> DPDTAVTNKQSFSTDVIYQVFTDRFLDGNPSNNPTGAAYDATCSNLKLYCGGDWQGLINKINDNYFSDLGVTALWISQPVENIFATINYSGVTNTAYHGYWARDFKKTNPYFGTMADFQNLITTAHAKGIKIVIDFAPNHTSPAMETDTSFAENGRLYDNGTLVGGYTNDTNGYFHHNGGSDFSSLENGIYKNLYDLADFNHNNATIDKYFKDAIKLWLDMGVDGIRVAAVKHMPLGWQKSWMSSIYAHKPVFTFGEWFLGSAASDADNTDFANKSGMSLLDFRFNSAVRNVFRDNTSNMYALDSMINSTATDYNQVNDQVTFIDNHDMDRFKTSAVNNRRLEQALAFTLTSRGVPAIYYGTEQYLTGNGDPDNRAKMPSFSKSTTAFNVISKLAPLRKSNPAIAYGSTQQRWINNDVYVYERKFGKSVAVVAVNRNLSTSASITGLSTSLPTGSYTDVLGGVLNGNNITSTNGSINNFTLAAGATAVWQYTTAETTPTIGHVGPVMGKPGNVVTIDGRGFGSTKGTVYFGTTAVTGAAITSWEDTQIKVTIPSVAAGNYAVKVAASGVNSNAYNNFTILTGDQVTVRFVVN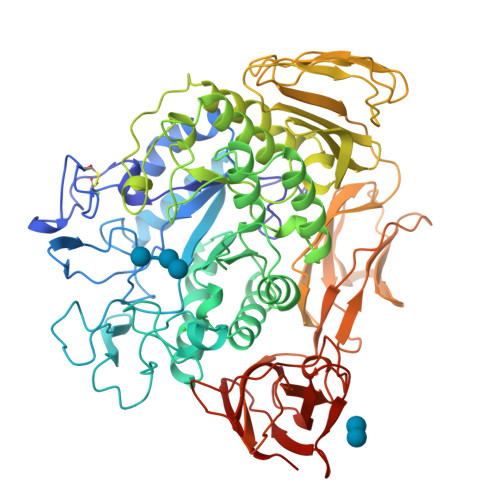NASTTLGQNLYLTGNVAELGNWSTGSTAIGPAFNQVIHQYPTWYYDVSVPAGKQLEFKFFKKNGSTITWESGSNHTFTTPASGTATVTVNWQ>XAAKDLLKADDIKKALDAVKAEGSFNHKKFFALVGLKAMSANDVKKVFKAIDADASGFIEEEELKFVLKSFAADGRDLTDAETKAFLKAADKDGDGKIGIDEFETL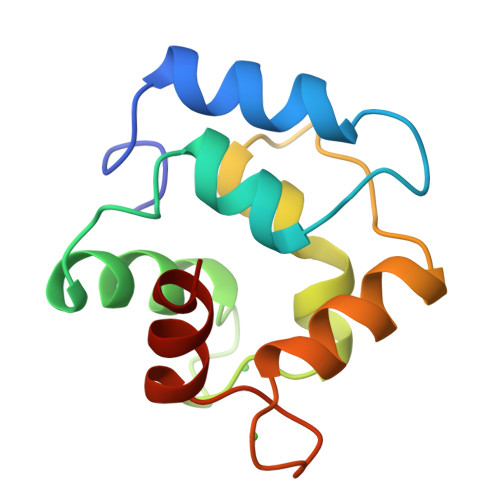VHEA[2x]>[8x]MARFEEQKLYIGGRYVEASSGATFETINPANGEVLAKVQRASREDVERAVQSAVEGQKVWAAMTAMQRSRILRRAVDILRERNDELAALET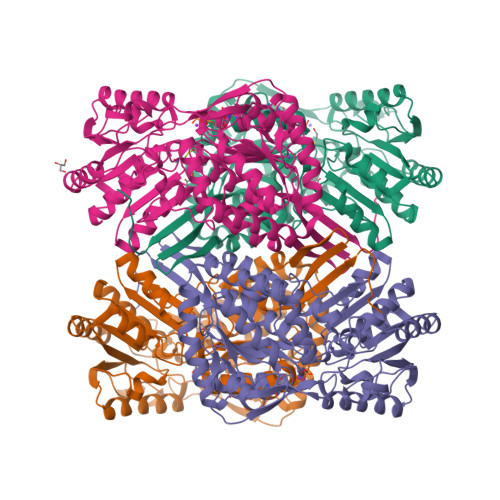LDTGKPLAETRSVDIVTGADVLEYYAGLVPAIEGEQIPLRETSFVYTRREPLGVVAGIGAWNYPVQIALWKSAPALAAGNAMIFKPSEVTPLTALKLAEIYTEAGVPDGVFNVLTGSGREVGQWLTEHPLIEKISFTGGTSTGKKVMASASSSSLKEVTMELGGKSPLIIFPDADLDRAADIAVMANFFSSGQVCTNGTRVFIHRSQQARFEAKVLERVQRIRLGDPQDENTNFGPLVSFPHMESVLGYIESGKAQKARLLCGGERVTDGAFGKGAYVAPTVFTDCRDDMTIVREEIFGPVMSILVYDDEDEAIRRANDTEYGLAAGVVTQDLARAHRAIHRLEAGICWINTWGESPAEMPVGGYKQSGVGRENGLTTLAHYTRIKSVQVELGDYASVF>GSHMNPLASLTTDKNDLYINWLKSLSFFQTNSSCAEALVKVIPHYHNKLIDFSQVLQLVFSASEKFPIQENQPLPEQLMFLSNLEKQT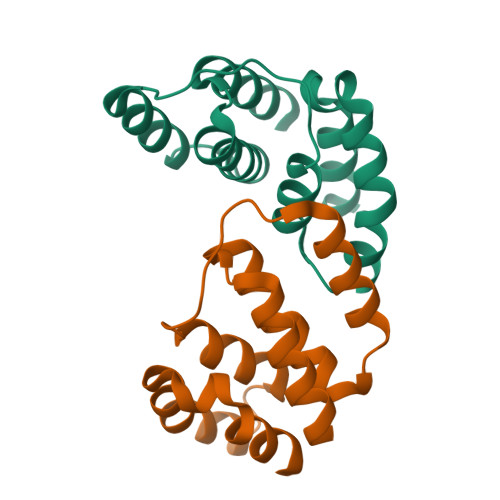PFAKAVGSSIYKLVTGKNLSLDFASQILKEASILEH[3x]N-(1H-benzimidazol-1-yl)-2-phenylacetamide | C15 H13 N3 O | 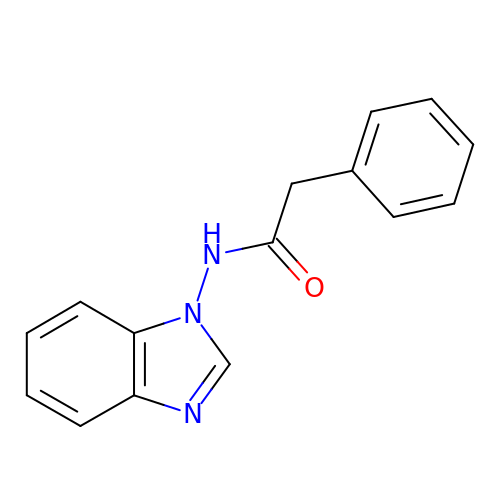LGOMVYVBROQGHX-UHFFFAOYSA-N> QANLMRLKSDLFNRSPMYPGPTKDDPLTVTLGFTLQDIVKVDSSTNEVDLVYYEQQRWK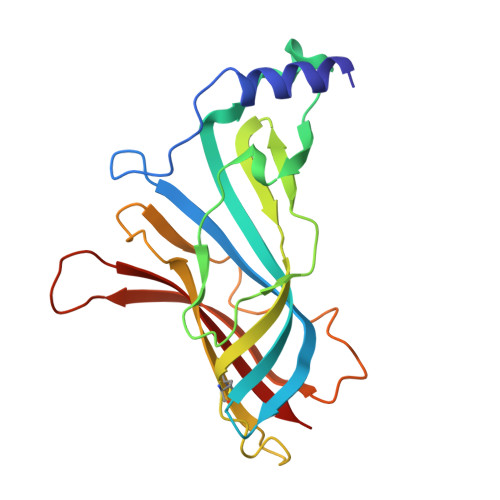LNSLMWDPNEYGNITDFRTSAADIWTPDITAYSSTRPVQVLSPQIAVVTHDGSVMFIPAQRLSFMCDPTGVDSEEGVTCAVKFGSWVYSGFEIDLKTDTDQVDLSSYYASSKYEILSATQTRQVQHYSCCPEPYIDVNLVVKFRE>[2x]NLLEEESAVLGQAVTNLMLSGDNVNNKNIILSLIHSLETTSDI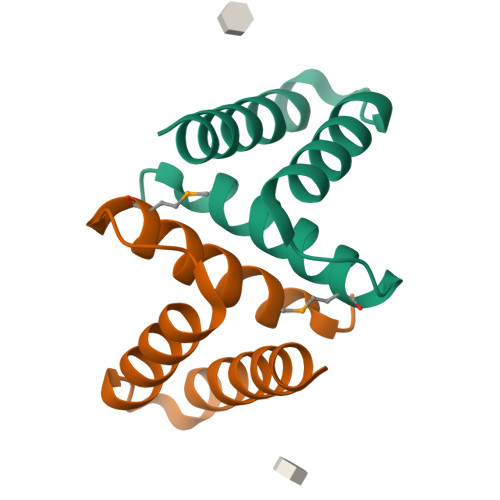LKADVIRKTLEIVLRYTADDM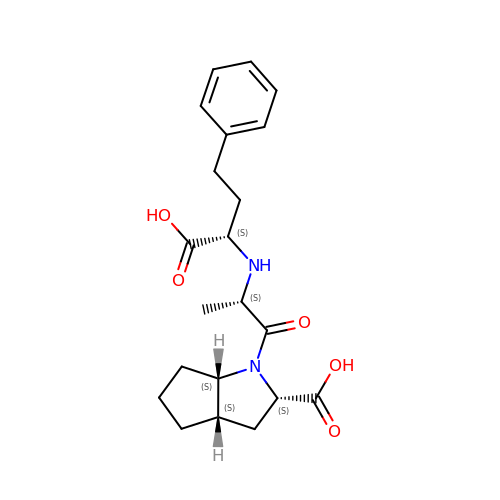Ramiprilat | C21 H28 N2 O5 | KEDYTOTWMPBSLG-HILJTLORSA-N Glycation, a non-enzymatic post-translational modification occurring on proteins, can be actively reversed via site-specific phosphorylation of the fructose-lysine moiety by FN3K kinase, to impact the cellular function of the target protein. Alternatively, the sugar moiety on glycated residues can be phosphorylated by a class of small-molecule kinases called fructosamine-3-kinases (FN3Ks), which are present in mammals, birds, and plants. Further characterization indicated that FN3K is responsible for protein deglycation by phosphorylating protein-associated fructosamines. Here, we determined a series of crystal structures of HsFN3K in the apo-state, and in complex with different nucleotide analogs together with a sugar substrate mimic to reveal the features important for its kinase activity and substrate recognition.

To gain molecular insights into the post-catalytic state of FN3K, we sought to capture HsFN3K with a phosphorylated substrate in its binding site. We mutated Asp217 to a serine residue to create extra space for the phosphate while maintaining the overall negative charge in the binding pocket. We obtained crystals of the HsFN3K∆_D217S variant in its apo form and performed soaking experiments using a mixture of an enzymatically prepared phosphorylated-DMF and ADP. The overall kinase fold in this structure is almost identical to our previously described HsFN3K∆ structures, but the N-lobe α1-helices are not swapped in this structure, likely due to the different crystallization condition for HsFN3K∆_D217S. Interestingly, in the nucleotide-binding site, a clear density for ATP (unused ATP from the mix containing phosphorylated-DMF) was observed in both protomers in the asymmetric unit with a flipped Trp219 binding its γ-phosphate. The empty substrate binding site indicates that either the phosphorylated-DMF is too unstable to be trapped in the crystal or that the D217S mutation is unable to stabilize the phospho-DMF, which diffuses out of the binding site. Furthermore, a serine would be too far to H-bond with the O3’ of the sugar moiety, explaining why DMF is absent in the substrate binding site in this structure. Notably, in the HsFN3K-D217S structure, the distance between the nitrogen of the flipped W219 side chain and ATP γ-phosphate increases by ~0.5 Å compared to the HsFN3K-ATP structure, due to the slight movement in the γ-phosphate positioning in the absence of the sugar moiety in the substrate binding site. This observation suggests that sugar binding also influences the nucleotide geometry in the binding site, and a true pre-steady state would not be attained in the absence of the substrate sugar in HsFN3K.

>[2x]AMEQLLRAELRTATLRAFGGPGAGCISEGRAYDTDAGPVFVKVNRRTQARQMFEGEVASLEALRSTGLVRVPRPMKVIDLPGGGAAFVMEHLKMKSLSSQASKLGEQMADLHLYNQKGSSYVDKFGFHTVTCCGFIPQVNEWQDDWPTFFARHRLQAQLDLIEKDYADREARELWSRLQVKIPDLFCGLEIVPALLHGSLWSGNVAEDDVGPIIYDPASFYGHSEFELAIALMFGGFPRSFFTAYHRKIPKAPGFDQRLLLYQLFNYLNHWNHFGREYRSPSLGTMRRLLK>[2x]VQLHKPDVVAAATKILDDHGIADLTMRRLARELD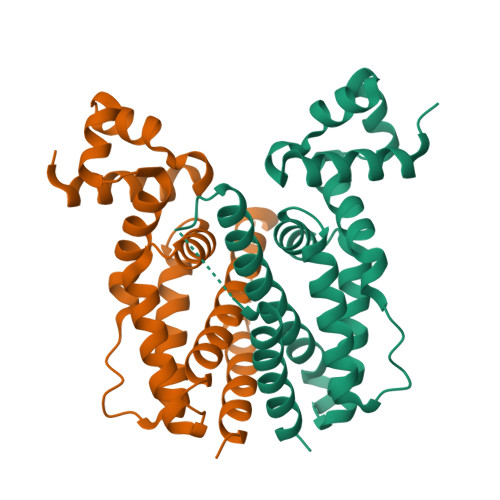VTPGALYWHFANKQELLGAVADHILRTARTDTADLAWREQIHESCRALRDALLSHTDGAELVSASFASGQSVVITEIVEQLGRAARAAGVSDADVDAAARTVIYYVLGFTVDEQSRLQWDAVGALGDDQSMLTRDGTRQFRFGLQLLVDGLAAHGGGSEFTGFSSAERSFE> GAMGSGIRVHHIKRRDIVLKWELGEGAFGKVFLAECHNLLPEQDKMLVAVKALKEASESARQDFQREAELLTMLQHQHIVRFFGVCTEGRPLLMVFEYMRHGDLNRFLRSHGPDAKLLAGGEDVAPGPLGLGQLLAVASQVAAGMVYLAGLHFVHRDLATRNCLVGQGLVVKIGDFGMSRDIYSTDYYRVGGRTMLPIRWMPPESILYRKFTTESDVWSFGVVLWEIFTYGKQPWYQLSNTEAIDCITQGRELERPRACPPEVYAIMRGCWQREPQQRHS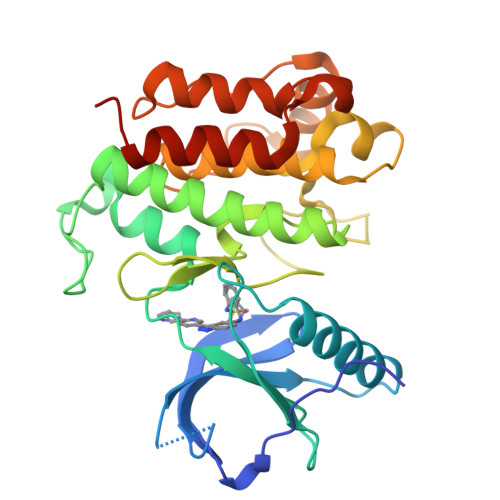IKDVHARLQALAQAPPVYLDVLG> MHHHHHHQGSVTEFLKPRLVDIEQVSSTHAKVTLEPLERGFG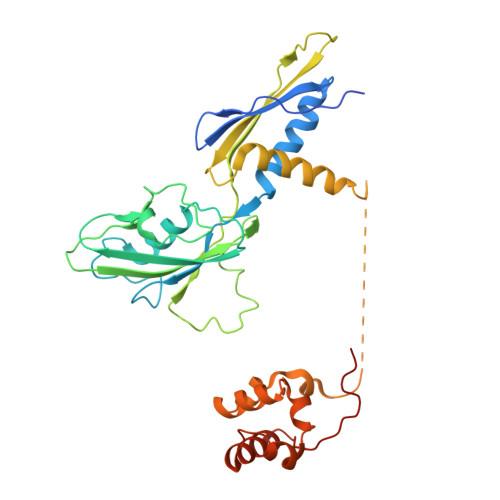HTLGNALRRILLSSMPGCAVTEVEIDGVLHEYSTKEGVQEDILEILLNLKGLAVRVQGKDEVILTLNKSGIGPVTAADITHDGDVEIVKPQHVICHLTDENASISMRIKVQRGRGYVPASTRIHSEEDERPIGRLLVDACYSPVERIAYNVEAARVEQRTDLDKLVIEMETNGTIDPEEAIRRAATILAEQLEAFVDLRDVRQPEVKEEKPEFDPILLRPVDDLELTVRSANCLKAEAIHYIGDLVQRTEVELLKTPNLGKKSLTEIKDVLASRGLSLGMRLENWPPASIADE>[15x]MAVKGLGEVDQKYDGSKLRIGILHARWNRKIIDALVAGAVKRLQEFGV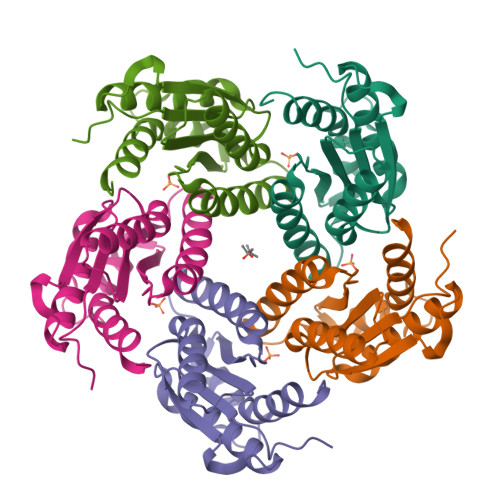KEENIIIETVPGSFELPYGSKLFVEKQKRLGKPLDAIIPIGVLIKGSTMHFEYICDSTTHQLMKLNFELGIPVIFGVLTCLTDEQAEARAGLIEGKMHNHGEDWGAAAVEMATKFN> FDNPPTNVVSHLNGDWFLFGDARSDCNHVVNTNPRNYSYMDLNPALCDSGKISSKAGNSIFRSFHFTDFYNYTGEGQQIIFYEGVNFTPYHAFKCTTSGSNDIWMQNKGLFYTQVYKNMAVYRSLTFVNVPYVYNGSAQSTALCKSGSLVLNNPAYIAREANFGDYYYKVEADFYLSGCDEYIVPLCIFNGK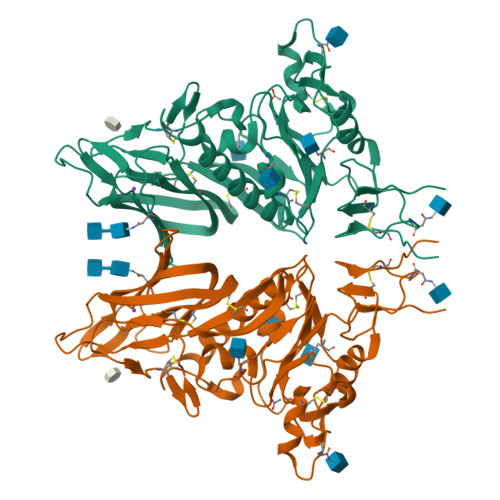FLSNTKYYDDSQYYFNKDTGVIYGLNSTETITTGFDFNCHYLVLPSGNYLAISNELLLTVPTKAICLNKRKDFTPVQVVDSRWNNARQSDNMTAVACQPPYCYFRNSTTNYVGVYDINHGDAGFTSILSGLLYDSPCFSQQGVFRYDNVSSVWPLYSYGRCPTAADINTPDVPICVYDSDPLVPR> SGVSSPAPCPAPCACDLDGGADCSGKGLVTVPDGLSVFTHSLDLSMNNITKLPEGAFKGFPYLEELRLAGNDLSIIHPMALSGLKELKVLTLQNNQLKTVPSESLKGLVSLQSLRLDANHIVTVPEDSFEGLVQLRHLWLDDNSLTEVPIRPLSNLPSLQALTLALNKISHIPDYAFSNLSSLVVLHLHNNKIRTLGPHSFHGLDNLEALDLNYNNLIDFPDSIRSLPNLKELGFHSNSITIIPDGAFVKNPLLRTIHLYDNPLSFVGNSAFQNLSDLHFLIIRGASNVQWFPNLTGTNNLESLTLTGTKIRSIPIKFCQEQKMLRTLDLSYN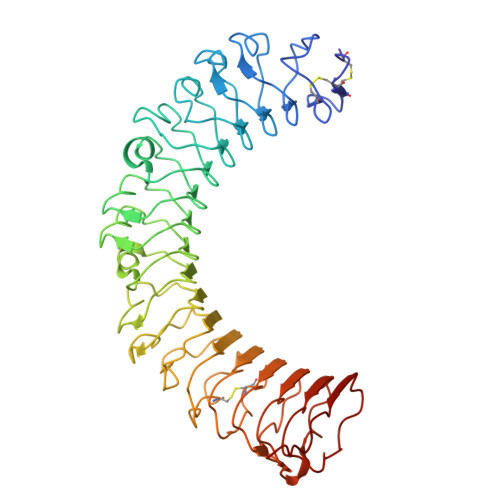EISALVGFEGCSSLEEVYLQNNQIQEVQNETFQGLAALRMLDLSRNRIHTIHKEAFVTLKALTNLDLSFNDLTAFPTAGLHGLNQLKLTGNPNFKETLT> MVKVGGEAGPSVTLPCHYSGAVTSMCWNRGSCSLFTCQNGIVWTNGTHVTYRKDTRYKLLGDLSRRDVSLTIENTAVSDSGVYCCRVEHRGWFNDMKITVSLEIVPP

TIM family proteins exhibit a classical type I membrane protein structure with an N-terminal immunoglobulin variable Ig-like (Ig V) domain, a heavily O-linked-glycosylated mucin-like domain (MLD) and a short C-terminal cytoplasmic tail. Recent studies indicate that hTIM-1, with some other but not all phosphatidylserine (PS) binding receptors, functions as a common attachment factor for a range of enveloped viruses, including filoviruses, flaviviruses, HIV, etc., through direct interaction with PS of the viral envelope. The Ig V domains of hTIM-1 and hTIM-4, exhibit two antiparallel β sheets with the front and back faces formed by A, G, F, C, C′, C″ and B, E, D strands respectively. A hydrophobic cleft formed by CC’ and FG loops, located at an equivalent position in hTIM-1 and hTIM-4 structures represents the putative PS ligand binding site.

We crystallized the Ig V domains of hTIM-1 and hTIM-4 and determined the structures at a resolution of 1.3 Å and 2.3 Å, respectively, using the molecular replacement method. While hTIM-1 has only one molecule in the asymmetric unit, there are eight molecules of essentially the same structure present in the asymmetric unit of hTIM-4. Despite sharing overall structural similarities with other Ig V domains of TIM family proteins, hTIM-1 Ig V domain exhibits unique features that may be essential for its distinct biological roles. Most notably, hTIM-1 possesses a significantly short BC loop that is the most variable structural feature amongst Ig V domains of the TIM family. In addition the residues of BC loop carry smaller side chains when compared to other TIM family proteins. This structural feature coupled with the movement of FG loop of hTIM-1 away from the BC loop, creates a unique groove that merges with the PS binding cleft. Two residues (Arg 110 and Arg 86) in hTIM-1 (while the counterparts are Pro and Gly, respectively in other TIM family members) render the two walls of the groove positively charged. We show that the Ig V domain of hTIM-1, but not other TIM family members, interacts directly with the GP and more specifically with the RBD of EBOV in vitro. In addition, the single mutations R86/A86 and R110/A110, exhibiting 60% and 50% reduction, respectively, in the binding affinity of hTIM-1 to Ebola GP, confirmed the structural interpretation that the unique groove in hTIM-1 also participates in GP binding. Based on the above results, we conclude that all the three loops, BC, CC’ and FG, of hTIM-1 together constitute the binding sites to Ebola GP, of which the residues Arg 106, Trp 112, Phe 113, Asn 114, Asp 115 and Lys 117 are critically important for Ebola GP binding, while, the residues Arg 86, Arg 110 have moderate effects on GP binding. Additionally, we further identified a number of residues on these three loops, which are critical for the EBOV GP binding.1-nitrohexane | C6 H13 N O2 | 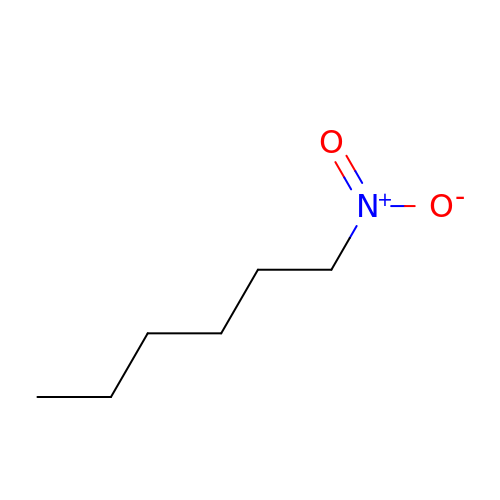FEYJIFXFOHFGCC-UHFFFAOYSA-N>ICLQKTTSTILKPRLISYTLPINTREGVCITDPLLAVDNGFFAYSHLEKIGSCTRGIAKQRIIGVGEVLDRGDKVPSMFMTNVWTPPNPSTIHHCSSTYHEDFYYTLCAVSHVGDPILNSTSWTESLSLIRLAVRPKSDSGDYNQKYIAITKVERGKYDKVMPYGPSGIKQGDTLYFPAVGFLPRTEFQYNDSNCPIIHCKYSKAENCRLSMGVNSKSHYILRSGLLKYNL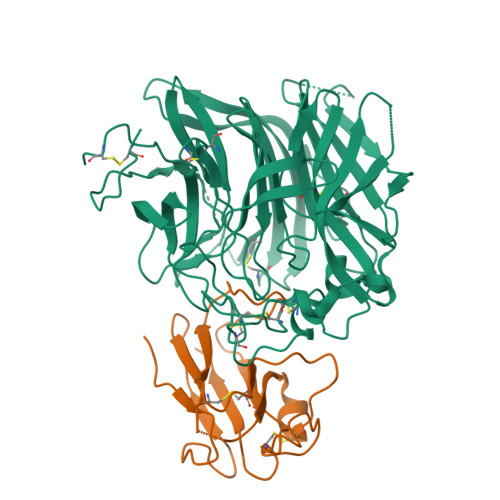SLGGDIILQFIEIADNRLTIGSPSKIYNSLGQPVFYQASYSWDTMIKLGDVDTVDPLRVQWRNNSVISRPGQSQCPRFNVCPEVCWEGTYNDAFLIDRLNWVSAGVYLNSNQTAENPVFAVFKDNEILYQVPLAEDDTNAQKTITDCFLLENVIWCISLVEIYDTGDSVIRPKLFAVKIPAQCSE[2x];>IVLEPIYWNSSNSKFLPGQGLVLYPQIGDKLDIICPKVDSKTVGQYEYYKVYMVDKDQADRCTIKKENTPLLNCAKPDQDIKFTIKFQEFSPNLWGLEFQKNKDYYIISTSNGSLEGLDNQEGGVCQTRAMKILMKVG[2x]>MGHHHHHHAKAVAPTTGWKQENGMWYFYNTDGSMATGWVQVNGSWYYLNSNGSMKVNQWFQVGGKWYYVNTSGELAVNTSIDGYRVNDNGEWVR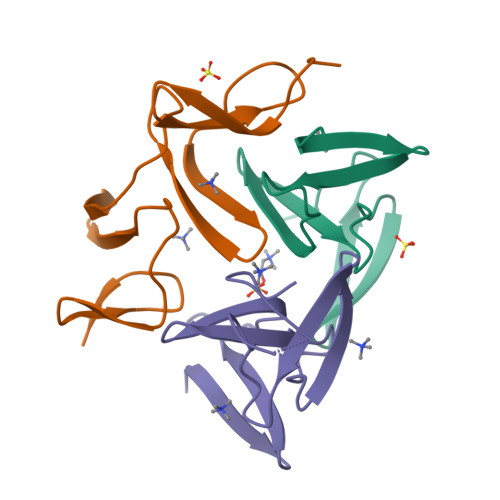[3x]> SSDQLLVDRTTNQLYVMLPGSNQLRPVYNLTSARLVLGNASNPVAVKSEELNRISKGQSIGIPGAPYATPTGTPASQWTLCDTVAKPDSSAPKVETSILIRTLAIDSGVGPIRADQGMLVSYEGANWLITEGGRHSIDLADRAVTSAVGIPVTAKPTPISQGLFNALPNRGPWQLPQIPAAGAPNSVGLPENLVIGSVFRTATESDPQHYVVLPDGVARVNNTTAAALRATNSYGLMQPPAVEASVVAKIPEQVYVSPLPDQPLDVLLRQDSPVLCWSWQREPGDQAPKTTVIAGRRLPLPANAIGTGIDQIGGDSTVYIEGGQFVRLQSPDPRVGESMYYIDPQGVRYGIANDDAAKNLGLAGPV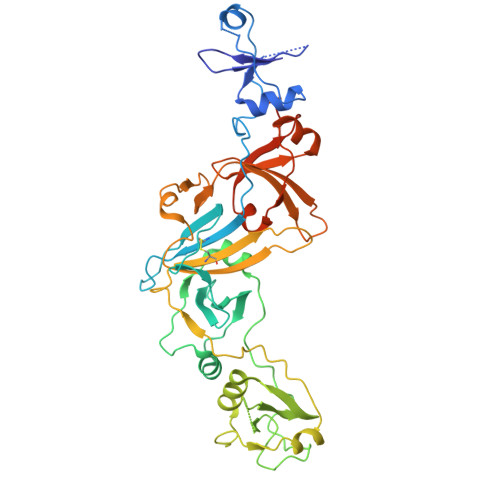NAPWQVVGLLVDGPVLSKEAALIEHDTLPADPNPRKVASGEG> KDIKKQITDINYLLLKNEEYKKYDIKKYNFFSSGKKINKGNIHLLTKQMRTFKEIFFSLGFEEMETHNYVESSFWC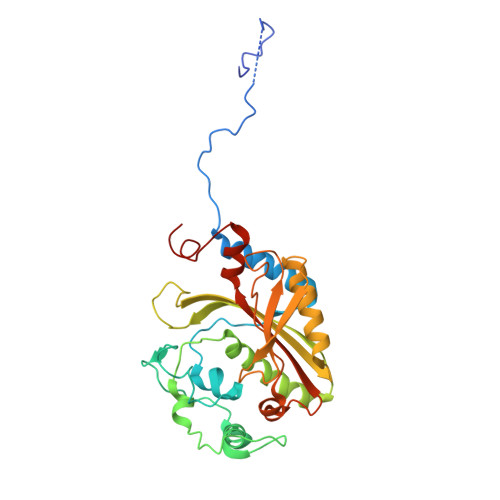FDALYIPQQHPSRDLQDTFFIKEPETCIDKFVDTEYIDNIKRVHTHGDYGSFGWNYKWKLEESKKNVLRTHTTANSCRALFKLAKEYKEAGCIKPKKYFSIDRVFRNENLDSTHLAEFHQVEGLIIDKNIGLSHLIGTLAAFYKHIGIHKLKFKPTFNPYTEPSMEIYGYHEQSKKWLEVGNSGIFRPEMLRSMGFSEEVSVIAWGLSLERPTMIKYNIKNIRDLFGYKSVV>[2x]MIKVYRYEIVKPLDLDWKEFGTILRQLQQETRFALNKATQLAWEWMGFSSDYKDNHGEYPKSKDILGYTNVHGYAYHTIKTKAYRLNSGNLSQTIKRATDRFKAYQKEILRGDMSIPSYKRDIPLDLIKENISVNRMNHGDYIASLSLLSNPAKQEMNVKRKISVIIIVRGAGKTIMDRILSGEYQVSASQIIHDDRKNKWYLNISYDFEPQTRVLDLNKIMGIAL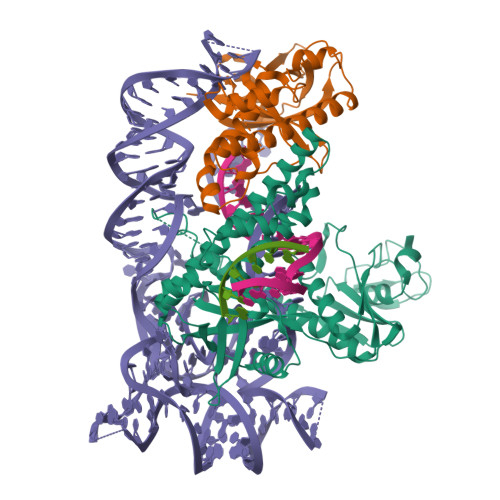GVAVAVYMAFQHTPARYKLEGGEIENFRRQVESRRISMLRQGKYAGGARGGHGRDKRIKPIEQLRDKIANFRDTTNHRYSRYIVDMAIKEGCGTIQMEDLTNIRDIGSRFLQNWTYYDLQQKIIYKAEEAGIKVIKIDPQYTSQRCSECGNIDSGNRIGQAIFKCRACGYEANADYNAARNIAIPNIDKIIAESIK> SNAMSIESSATPTTPNAEALQLNSTEVRILGCLIEKQATNPETYPLTLNALVIACNQKTSRDPVMNLTQGQVGQSLRALEGRGLTRLVMGSRADRWEHKVDKGLELVPAQVILTGLLLLRGPQTVSELLTRSNRMHDFEDSEQVVHQLERLIARGLATLVPRQSGQREDRY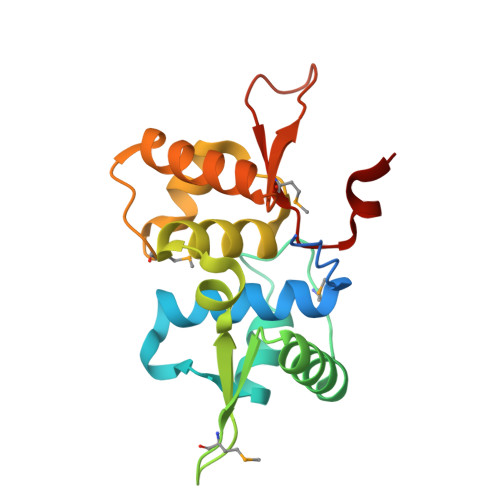MHLIGDPEDLQD>MSDTMVVNGSGGVPAFLFSGSTLSSYRPNFEANSITIALPHYVDLPGRSNFKLMYIMGFPIDTEMEKDSEYSNKIRQESKISKTEGTVSYEQKITVETGQEKDGVKVYRVMVLEGTIAESIEHLDKKENEDILN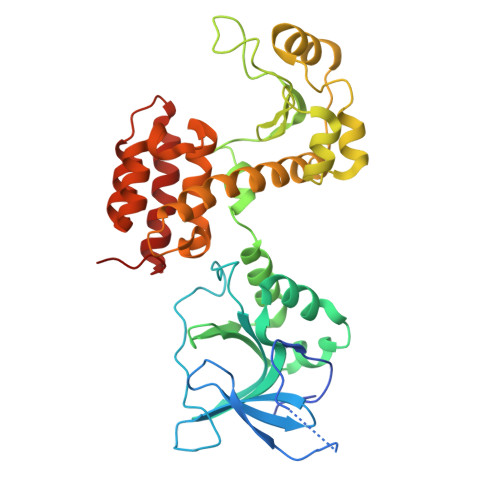NNRNRIVLADNTVINFDNISQLKEFLRRSVNIVDHDIFSSNGFEGFNPTSHFPSNPSSDYFNSTGVTFGSGVALGQRSKQDLLNDGVPQYIADRLDGYYMLRGKEAYDKVRTAPLTLSDNEAHLLSNIYIDKFSHKIEGLFNDANIGLRFSDLPLRTRTALVSIGYQKGFKLSRTAPTVWNKVIAKDWNGLVNAFNNIVDGMSDRRKREGALVQKDIDSGLLKLE[2x]The active ingredient of Bti is a parasporal body that contains three natural sub-micron-sized crystals of four highly efficient mosquito-specific toxins, namely Cyt1Aa, Cry11Aa and co-crystallizing Cry4Aa and Cry4Ba. Following ingestion by mosquito larvae, the crystals promptly dissolve in the alkaline environment of the gut (pH ~11), releasing protoxins that are activated into toxins through proteolytic cleavage of propeptides by gut enzymes. Each activated protein eventually self-assembles into cytolytic oligomers that perforate gut cells, leading to mosquito larvae death. Here, we use serial femtosecond crystallography (SFX) at an X-ray free electron laser (XFEL) to identify the features governing the in vivo crystallization of Cyt1Aa in Bti cells, and to track the structural dynamics driving natural crystal dissolution in the alkaline mosquito larvae gut.

We engineered a C7S mutation to probe the role of the disulfide bridge. By recombinant expression in Bti-4Q7, we obtained sub-micron-sized crystals diffracting to 2.0 Å resolution, which revealed a structure nearly indiscernible from the “DTT” structure. Thus, neither crystal formation nor crystalline order depends on the disulfide-bridge chaining of DS dimers. This step therefore likely occurs after the crystal is fully formed. In contrast, the C7S crystals dissolve in the absence of DTT at the same pH as WT crystals soaked with DTT and remain unperturbed by addition of DTT. Hence, the disulfide bridge contributed by C7 increases the resilience of WT crystals by diminishing their pH sensitivity. The disulfide-bridged dimer is unable to form MBO upon contact with liposomes (~100 nm radius; LUVs) whereas the C7S mutant, able only to solubilize as protoxin monomers, forms MBO regardless of proteolytic activation. The C7S, C190V and Y171F mutants, which form MBO, display the same toxicity as the WT, excluding a possible role for these residues in cytolytic oligomer formation.

> MENLNHSPLEDIKVNPWKTPQSTARVITLRVEDPNEINNLLSINEIDNPNYILQAIMLANAFQNALVPTSTDFGDALRFSMPKGLEIANTITPMGAVVSYVDQNVTQTNNQVSVMINKVLEVLKTVLGVALSGSVIDQLTAAVTNTFTNLNTQKNEAWIFWGKETANQTNYTYNVLFAIQNAQTGGVMYCVPVGFEIKVSAVKEQVLFFTIQDSASYNVNIQSLKFAQPLVSSSQYPIADLTSAINGTL> SNAMPAPSSPRKNQTSFDPEMLLKLVTDSLDDDQALEIATIPLAGKSSIADYMVIASGRSSRQVTAMAQKLADRIKAATGYVSKIEGLPAADWVLLDAGDIIIHLFRPEVRSFYNLERMWGFGDE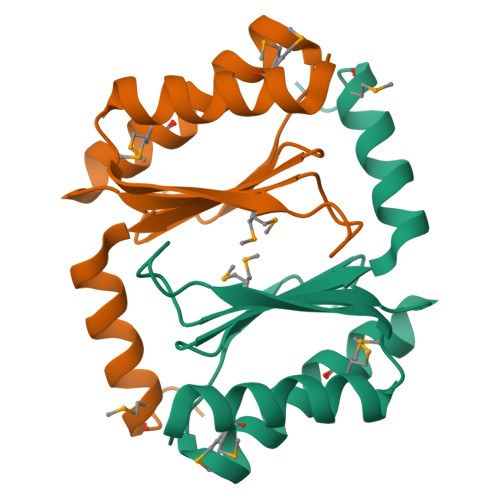SDQPVSQSVLS Three receptor types have been highlighted: VEGFR3 (also called Flt-4) regulates lymphangiogenesis, VEGFR2 (KDR/Flk-1) is the primary proangiogenic receptor, whereas VEGFR1 (Flt-1) has been proposed as a regulator of VEGFR2. In this study, we showed the presence of a metal site at the dimer interface of X-ray structures of human VEGFR1 domain 2 (hVEGFR1d2) solved in the presence of different divalent metal ions. The three structures are similar and reveal a homodimer with interlocked hydrophobic surfaces buried at the interface and a divalent cation chelated by four histidine residues (two from each monomer). Importantly, the dimer interface involves residues that lie in the core of the hVEGFR1d2 surface that interacts with VEGF-A, VEGF-B or PlGF.

Although the presence of a ligand was not observed in the crystal structure, we observed the unexpected presence of one metal ion characterized as Zn2+ using X-ray fluorescence spectrometry. Contrary to the Co2+ and to the Cu2+ ions, the Zn2+ was not intentionally added in crystallization conditions, but was a posteriori identified by X-ray fluorescence. A zinc contamination arising from laboratory items cannot be excluded or from the putative ligand Laxaphycin B. This cyclic peptide does not possess the peculiarity of some Zn2+ chelating peptides as Cys residues, or thiazole and oxazoline rings. The Zn2+ ion adopted a regular tetrahedral coordination geometry and was coordinated through the Nε atoms of the imidazole groups of His147 and His223. The metal ion coordination site is octahedral for Co2+ and tetrahedral for Zn2+ and Cu2+. The mean estimation for ΔG dissociation was 12.7 kcal.mol-1, 58.1 kcal.mol-1 and 18.4 kcal.mol-1 for (hVEGFR1d2)2-Co2+, -Zn2+, and -Cu2+ respectively. Zn2+ and Ni2+ exhibited IC50 values within the micromolar range. To evaluate this hypothesis, a model of hVEGFR1d2d3 was built, oriented as in the VEGFR2d2d3 template and positioned as observed in the Zn2+ hVEGFR1d2 dimer structure, followed by a GROMOS molecular dynamics simulation performed in the presence of explicit water molecules and NaCl. The homodimeric model retains the d2 dimer interface and the bound Zn2+ ion after a 2 ns molecular dynamics simulation.

> GRPFVEMYSEIPEIIHMTEGRELVIPCRVTSPNITVTLKKFPLDTLIPDGKRIIWDSRKGFIISNATYKEIGLLTCEATVNGHLYKTNYLTHRQ In conclusion, we identified and characterized Paenibacillus spp. NagB1 and NagB2 proteins as SBPs for chitin oligosaccharides. Binding experiments of the recombinant NagB1 and NagB2 to several oligosaccharides using differential scanning fluorimetry and surface plasmon resonance confirmed that both proteins are SBPs of (GlcNAc)2 and (GlcNAc)3. SBPs, a component of ABC transporters, are responsible for trapping ligands that are imported through a specific pathway formed by two TMDs, and mainly define the specificity and affinity of transporters (Berntsson et al., 2010, ter Beek et al., 2014). The structures of NagB1 and NagB2 were classified as subcluster D-I and contained two α/β domains connected by a hinge region consisting of three strands, with the substrate-binding pocket located between the two domains.

The crystal structures of NagB2 in ligand-free or complex forms with (GlcNAc)2 (NagB2/(GlcNAc)2) and (GlcNAc)3 (NagB2/(GlcNAc)3) were determined at 1.2 to 1.8 Å resolution. There were two polypeptide chains in the asymmetric unit of the crystal of the ligand-free form (chain A, Asp47–Leu452 and chain B, Val49–Gly450), whereas there was only one polypeptide chain in the ligand-bound form. As indicated by the a.a. sequence similarity, the overall structure of NagB2 was very similar to that of NagB1, with an r.m.s.d. of 1.0 Å for the 394 Cα atoms between the (GlcNAc)2 bound forms. In the crystal structures, the bound oligosaccharides were confined at the binding sites in an extended conformation and were well defined in the density maps. In both (GlcNAc)2 bound structures of NagB1 and NagB2, the first GlcNAc interacted with the tryptophan residue Trp213 of NagB1 or Trp217 of NagB2 and formed hydrogen-bonding networks with surrounding residues. The O3, O4, O6, and O7 atoms of the first GlcNAc formed hydrogen bonds with Arg95, Asp401, and Ser330 of NagB1 and Arg96, Asp408, and Ser334 of NagB2. In NagB2/(GlcNAc)2, Lys416 interacted with the first GlcNAc via a water molecule. The second GlcNAc unit formed a CH/π interaction with Trp292 of NagB1 or Trp296 of NagB2. In NagB2, this residue was substituted with Thr65, but the spatially closer Arg373 played an important role in recognizing the second GlcNAc. When (GlcNAc)2 was bound, this angle changed to 56.8° between the closed and open forms and 30.2° between the closed and semi-closed forms.

> MGCGGTADKNPAGNNGDSAKPAETKSGDSVSLTLRHINVRDTAKNTLALLEKVVKKTEAEVPGATFKLDGVEDTVNRDVKLKAEMAAGKPPQIFNLFGGADTQNYAKAGHLLPLNDILKELGLEDKFFELREFTVDGKIYGLPEAGFVEGFYYNTKLFADAGITSAPKTWDEFTKALEALKAKNITPIALGGGSGDGWAINMLANSLFVATAGPEAQEGFAKGTTKWTDPAVLDGFKRLKDLKDKGYIDPNVLGLKYSEGQAKFYTGQAAMLFDGSWATSAILDKDKSTVKDNVGYFRFPNIGGKGDNLINGGWSNGYGFSSHLNDAEKKAVKAFIKNFYTLEIQGEALGRDNRVPSMKGVPTPAEAAPLTKAIGEAQASAKAAFPAFDALVQPKVKVTLEQSVQELLGGQLTPEKLVEKMQKVQDEANAGKLEHHHHHH> MGSWSHPQFEKSSGLVPRGSMTRRWYLCCSRHHLDTVPEDSDGIVVPVTEHGVATLLPRYPETYEVEDIVDVAKDRGLSVQALMDFTCAGCEHLSPDGYPSLRSTLDYLASDLEVDGVVVAD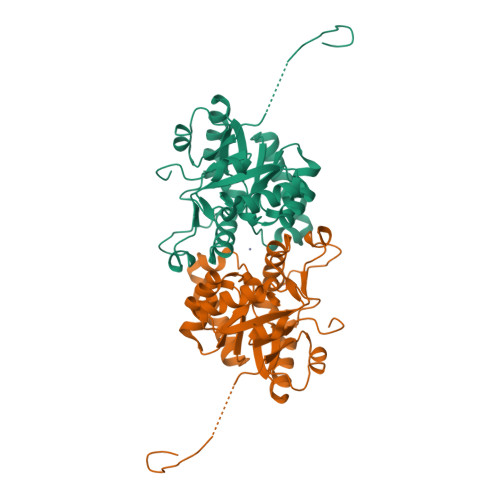PYLVEVLATEYDLTVVVSHTAAVDTPEKAWHFERLGADVITVDPALNSNEEEVSAIRERVSVELRTAVGAITFRDPVAFFERNLFSHATAEGIEVDPYRNNPYEPMRERVVVWEVREELFDEVFILASGEPP> MLPPDILQNGEFETIYFQTNPTYIKSPIHIPKSTIGKPDTVKIRHFFALLHQDLVVLGLEVFVYLQIYSDFVEKYVYVSKCDTVGLEKSTIKIGKVIGPVLQYIINYNGYKIKMKNLDEKSKDLSDPSTLVRLQRLRDKLPDIYPNLPYYN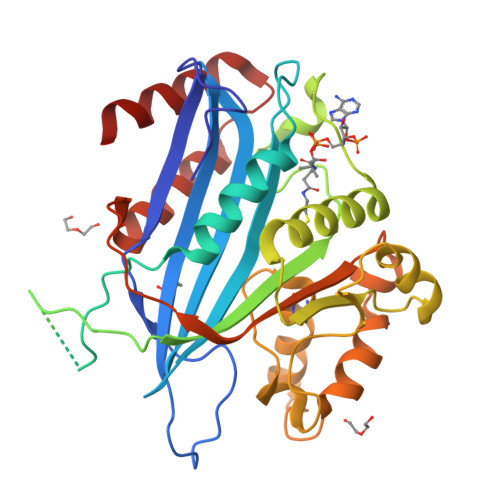DIPPKEECIEYRTLPKTQNLRLCVFTKPAKEYLFPNSAKNPYKNLLNGQSLLRWWISIIDSITKGWNNHKLMIPGADKWATRKFIEKYSDWSEGHIFKKDGLAVQAIPLFPDDPKGRFLELVIVECRYGKMTVSRFYQELAYRQEFLLGDCVSLIGCCKENLEVTYHDDLVSTVTISEYKEFMNLLKLVDFSDRVEVSNFVSNYRKSK>ATSSACPQYVLINTRGTGEPQGQSAGFRTMNSQITAALSGGTIYNTVYTADFSQNSAAGTADIIRRINSGLAANPNVCYILQGYSQGAAATVVALQQLGTSGAAFNAVKGVFLIGNPDHKSGLTCNVDSNGGT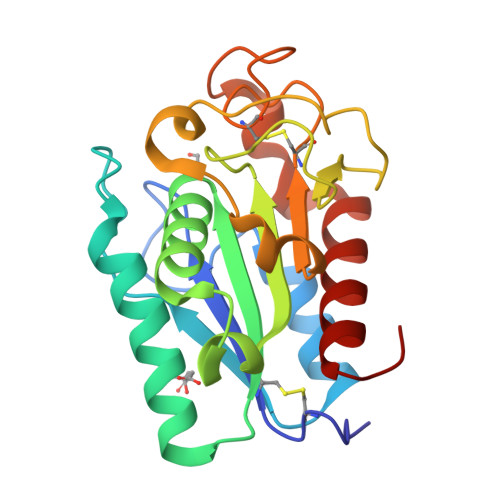TTRNVNGLSVAYQGSVPSGWVSKTLDVCAYGDGVCDTAHGFGINAQHLSYPSDQGVQTMGYKFAVNKLGGSA[2x]> MISDS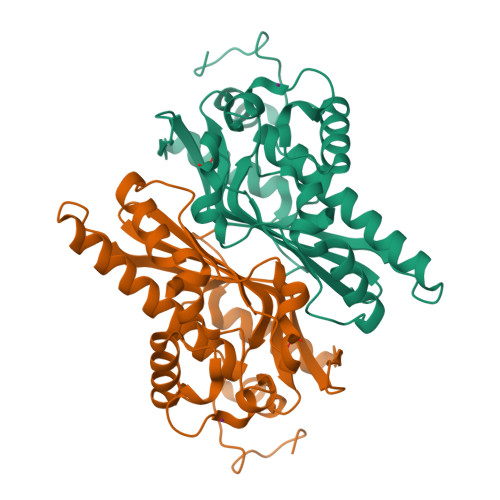MTVEEIRLHLGLALKEKDFVVDKTGVKTIEIIGASFVADEPFIFGALNDEYIQRELEWYKSKSLFVKDIPGETPKIWQQVASSKGEINSNYGWAIWSEDNYAQYDMCLAELGQNPDSRRGIMIYTRPSMQFDYNKDGMSDFMCTNTVQYLIRDKKINAVVNMRSNDVVFGFRNDYAWQKYVLDKLVSDLNAGDSTRQYKAGSIIWNVGSLHVYSRHFYLVDHWWKTGETHISKKDYVGKYA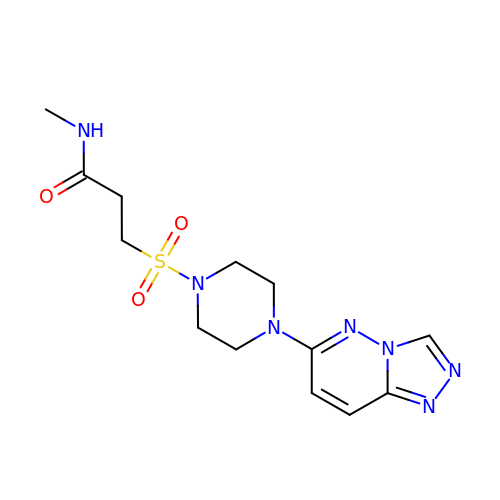~{N}-methyl-3-[4-([1,2,4]triazolo[4,3-b]pyridazin-6-yl)piperazin-1-yl]sulfonyl-propanamide | C13 H19 N7 O3 S | KVLQRUOLMVHSTQ-UHFFFAOYSA-N> MATLVLSSMPCHWLLFLLLLFSGEPVPAMTSSDLPLNFQGSPCSQIWQHPRFAAKKRSSMVKFHCYTNHSGALTWFRKRGSQQPQELVSEEGRIVQTQNGSVY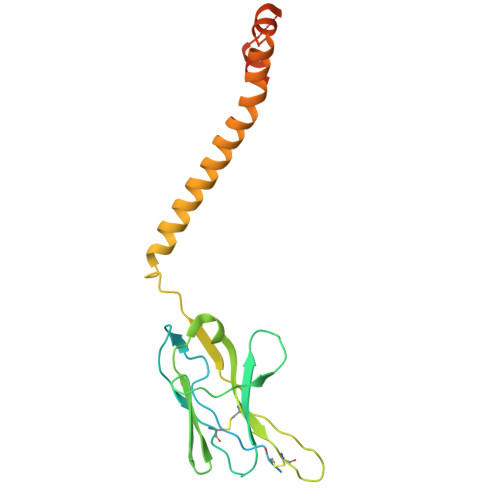TLTIQNIQYEDNGIYFCKQKCDSANHNVTDSCGTELLVLGFSTLDQLKRRNTLKDGIILIQTLLIILFIIVPIFLLLDKDDGKAGMEEDHTYEGLNIDQTATYEDIVTLRTGEVKWSVGEHPGQE>[4x]SEFENPLKRLLVPGEEWEFEVTAFYRGRQVFQQTISCPEGLRLVGSEVGDRTLPGWPVTLPDPGMSLTDRGVMSYVRHVLSCLGGGLALWRAGQWL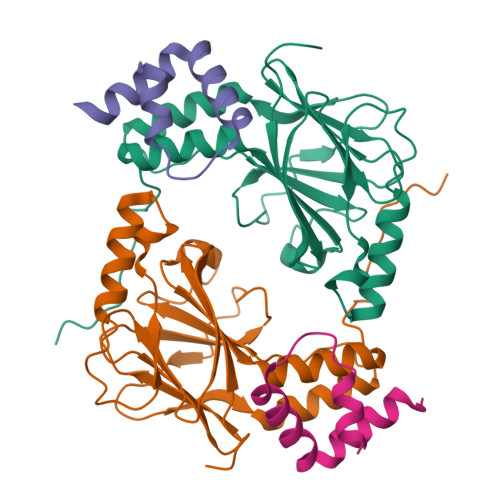WAQRLGHCHTYWAVSEELLPNSGHGPDGEVPKDKEGGVFDLGPFIVDLITFTEGSGRSPRYALWFCVGESWPQDQPWTKRLVMVKVVPTCLRALVEMARVGGASELENTVDLHIENS;>SALQDLLRTLKSPSSPQQQQQVLNILKSNPQLMAAFIKQRTAKYVAN[4x]>[2x]MGGSHHHHHHGENLYFQSVDDLTVEPNLHSLITSTTHKWIFVGGKGGVGKTTSSCSIAIQMALSQPNKQFLLISTDPAHNLSDAFGEKFGKDARKVTGMNNLSCMEIDPSAALKDMNDMAVSRANNNGSDGQGDDLGSLLQGGALADLTGSIPGIDEALSFMEVMKHIKRQEQGEGETFDTVIFDTAPTGHTLRFLQLPNTLSKL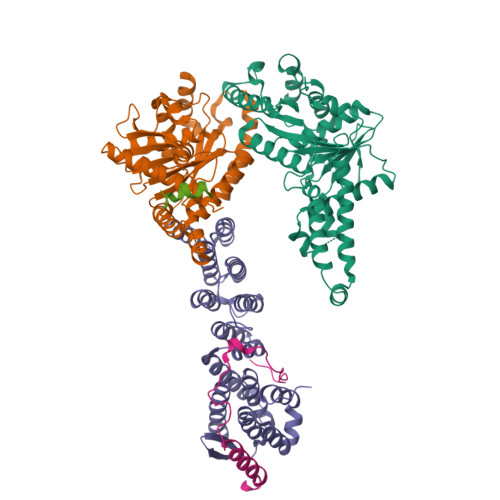LEKFGEITNKLGPMLNSFMGAGNVDISGKLNELKANVETIRQQFTDPDLTTFVCVCISEFLSLYETERLIQELISYDMDVNSIIVNQLLFAENDQEHNCKRCQARWKMQKKYLDQIDELYEDFHVVKMPLCAGEIRGLNNLTKFSQFLNKEYNPITDGKVIYELEDKE;> MVPAESNAVQAKLAKTLQRFENKIKAGDYYEAHQTLRTIANRYVRSKSYEHAIELISQGALSFLKAKQGGSGTDLIFYLLEVYDLAEVKVDDISVARLVRLIAELDPSEPNLKDVITGMNNWSIKFSEYKFGDPYLHNTIGSKLLEGDFVYEAERYFMLGTHDSMIKYVDLLWDWLCQVDDIEDSTVAEFFSRLVFNYLFISNISFAHESKDIFLERFIEKFHPKYEKIDKNGYEIVFFEDYSDLNFLQLLLITCQTADASYFLNLKNHYLDFSQAYKSELEFLGQEYFNENLYFQSLEHHHHHH;> MSTSASGPEHEFVSKFLTLATLTEPKLPKSYTKPLKDVTNLGVPLPTLKYKYKQ> SNMSW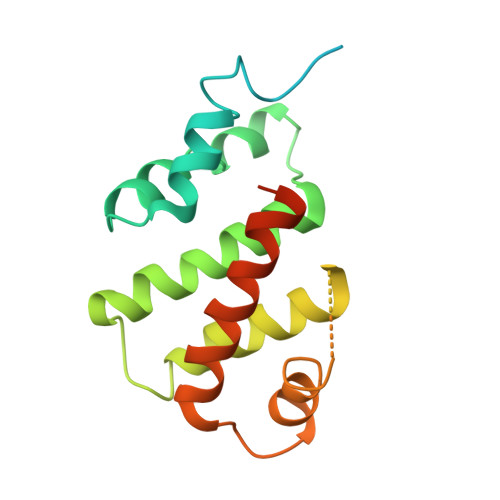ESGAGPGLGSQGMDLVWSAWYGKCVKGKGSLPLSAHGIVVAWLSRAEWDQVTVYLFCDDHKLQRYALNRITVWRSRSGNELPLAVASTADLIRCKLLDVTGGLGTDELRLLYGMALVRFVNLISERKTKFAKVPLKCLAQEVNIPDWIVDLRHELTHKKMPHINDCRRGCYFVLDWLQKTYWCRQLENSLRETWELE(3beta,14beta,17alpha)-ergosta-5,24(28)-dien-3-ol | C28 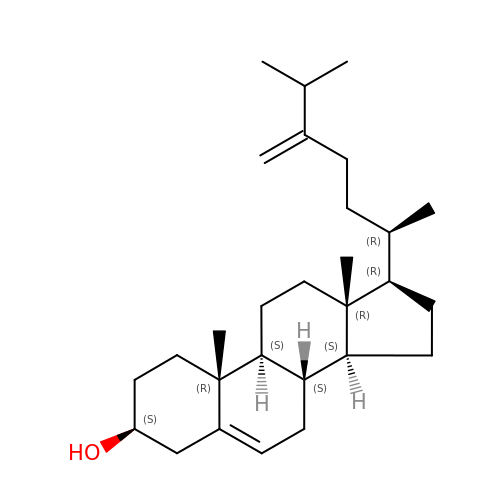H46 O | INDVLXYUCBVVKW-PXBBAZSNSA-N> EPQY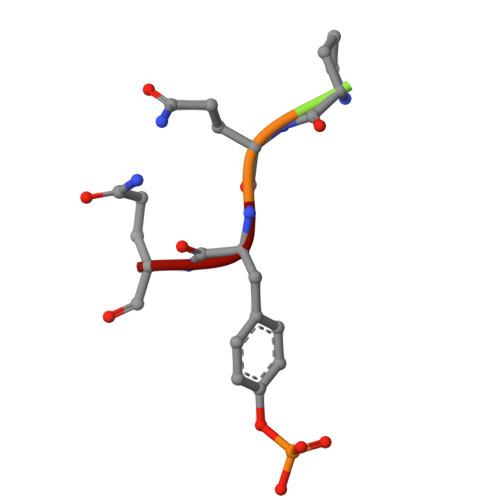Q> GPEFSLPQCINPFTNLPHTPRYYDILKKRLQLPVWEYKDRFTDILVRHQSFVLVGETGSGKTTQIPQWCVEYMRSLPGPKRGVACTQPRRVAAMSVAQRVADEMDVMLGQEVGYSIRFEDCSSAKTILKYMTDGMLLREAMNDPLLERYGVIILDEAHERTLATDILMG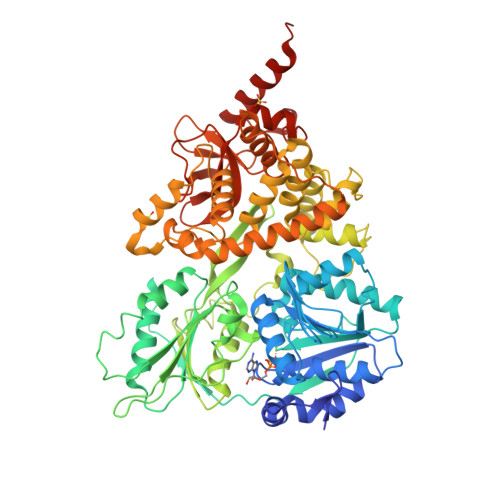VLKEVVRQRSDLKVIVMSATLDAGKFQIYFDNCPLLTIPGRTHPVEIFYTPEPERDYLEAAIRTVIQIHMCEEEEGDLLLFLTGQEEIDEACKRIKREVDDLGPEVGDIKIIPLYSTLPPQQQQRIFEPPPPKKQNGAIGRKVVVSTNIAETSLTIDGVVFVIDPGFAKQKVYNPRIRVESLLVTAISKASAQQRAGRAGRTRPGKCFRLYTEKAYKTEMQDNTYPEILRSNLGSVVLQLKKLGIDDLVHFDFMDPPAPETLMRALELLNYLAALNDDGDLTELGSMMAEFPLDPQLAKMVIASCDYNCSNEVLSITAMLSVPQCFVRPTEAKKAADEAKMRFAHIDGDHLTLLNVYHAFKQNHESVQWCYDNFINYRSLMSADNVRQQLSRIMDRFNLPRRSSDFTSRDYYINIRKALVTGYFMQVAHLERTGHYLTVKDNQVVQLHPSTVLDHKPEWVLYNEFVLTTKNYIRTCTDIKPEWLVKIAPQYYDMSNFPQCEAKRQLDRIIAKLQSKEYSQY>ARKCSLTGKWTDDLGSNMTIGAVNSRGEFTGTYITAVADNPGNITLSPLLGIQHKRASQPTFGFTVNWKFSESTTVFTGQCFIDRNGKEVLKTMWLLRSSVNDISDDWIATRVGINIFTRQRTQK[2x]

Common to all members of the avidin protein family is their high affinity towards a small ligand, D-biotin. Despite their relatively low amino acid sequence identity, all avidins share a highly similar tertiary structure, an eight-stranded β-sheet barrel structure, where the biotin-binding site is located at the open end of the barrel. With the exception of rhizavidin, shwanavidin and bradavidin II, all of the structurally characterized natural avidins are stable homotetramers with four biotin-binding sites, one on each monomer. We have previously created functional chimeric avidins using DNA shuffled sequences of AVD and avidin related protein 2 (AVR2).

Here, we present the crystal structure of the previously characterized chimeric mutant A/A2-1, which proves that the avidin fold is robust and suitable for extensive genetic manipulation. In addition, size exclusion chromatography indicated an oligomeric state smaller than a tetramer. Therefore, in order to better understand the structural origin of the physicochemical properties, the structure of mutant A/A2-1 was solved in complex with biotin at 1.8 Å resolution (see Table 1 for the structure determination statistics). Two monomers were found in the asymmetric unit and, as expected based on the high sequence identity to its parental proteins AVD and AVR2, the quaternary structure was homotetrameric, each monomer having an eight-stranded β-sheet barrel structure with the biotin-binding site located at the open end of the barrel. The sequence and structural differences to AVD are in the region derived from AVR2, starting at A38 of the L3,4-loop of A/A2-1 and ending with S58 of the L4,5-loop, whereas A/A2-1 differs from AVR2 at the N- and C-terminal regions originating from AVD. As observed in the crystal structure, D12 of A/A2-1 hydrogen bonds with the ureido oxygen of biotin in low pH conditions. A/A2-1 was crystallized at acidic conditions (pH near 4), and hence the X-ray structure of A/A2-1 represents a snapshot of conditions near the pKa of D12, where about 50% of the D12 residues in the crystal would be expected, if exposed to solvent, to be protonated. In the A/A2-1 structure the OD2 oxygen atom of D12 is surrounded by aromatic and nonpolar residues that would act to reduce the effective dielectric constant (in comparison to bulk water), effectively raising the pKa value and increasing the probability of a protonated D12. This would support the formation of a stable hydrogen bond at pH 4, thus explaining the hydrogen bond observed in the crystal structure. In the L3,4-loop of AVR2, AVR4 and A/A2-1, there is a proline residue, which introduces rigidity, and the loop is further stabilized by the intermonomeric salt bridge between D39 and R112 for A/A2-1 and reported earlier for AVR2 and AVR4.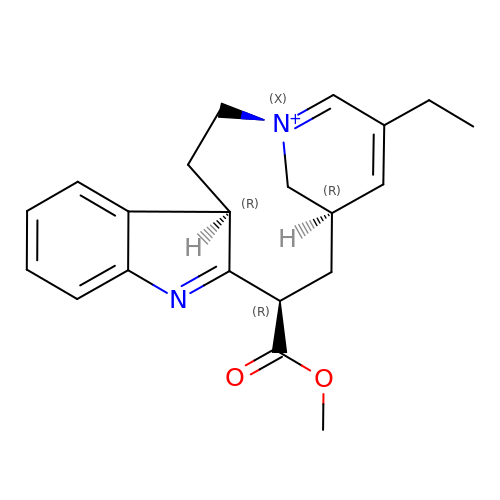18-carboxymethoxy-cleaviminium | C21 H25 N2 O2 | ULODILYUCKTWMV-CGTJXYLNSA-N L-BETA-ASPARTYLHISTIDINE 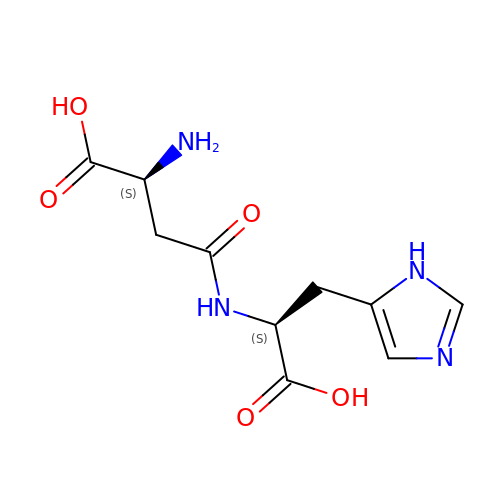| C10 H14 N4 O5 | KABYBYFUSGXITA-BQBZGAKWSA-N> MYWVRRKTIGGSGLPYTENEILEWRKEGVKRVLVLPEDWE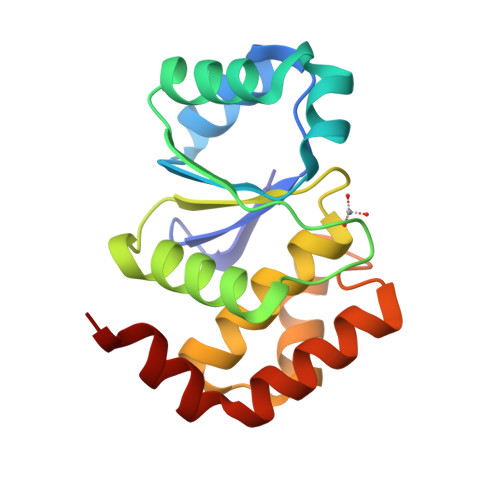IEESWGDKDYYLSILKKNGLQPLHIPIPDGGVPSDSQFLTIMKWLLSEKEGNLVHCVGGIGRTGTILASYLILTEGLEVESAIDEVRLVRPGAVQTYEQEMFLLRVEGMRKSWLKNIYSNS> AAAAAAAAAAAAAAAAAAAAAAAAAAAAAAAAAAAAAAAAAAAAAAAAAA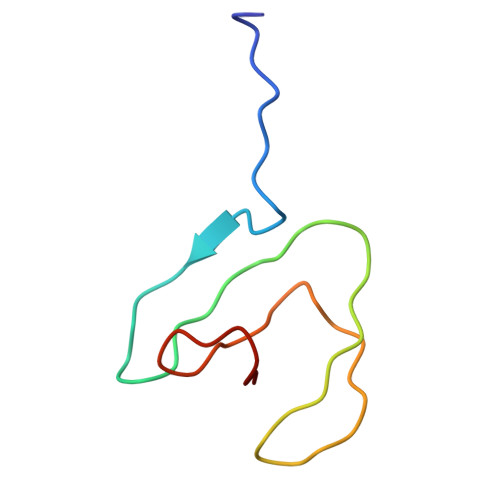AAAAAAAAA>[4x]SMSRPRILVPG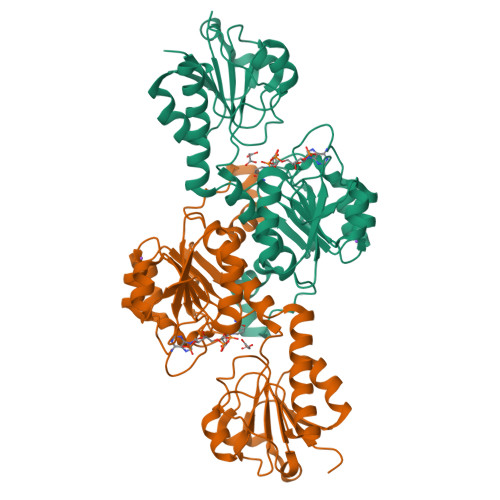KINPRVLERLPEMFETVRIERADAALVTADMRDVSGIAVSGKLPVPLMDAFPSLEIVANFGVGYDGVDVSRAAARGIVVTNTPDVLTEEVADTAIGLLLNTLRLLPQAEQWLRQGRWVREGAFPLSPLSLRGRTVGLFGLGRIGLAIARRLEAFGVSIAYHTRTPREGLGFTYHPTLVGMAEAVDTLIVIVPGTASTLKAVNADVLSALGPKGVLINVGRGSTVDEAALVTALQNGTIAGAGLDVFENEPNVPEALLSFPNVSLLPHVASASVVTRNAMSDLVVDNLKAWFSTGEALTPVAETPFRRRAIQN> MGHHHHHHLESTSLYKKSSSTPPRGVTVVNN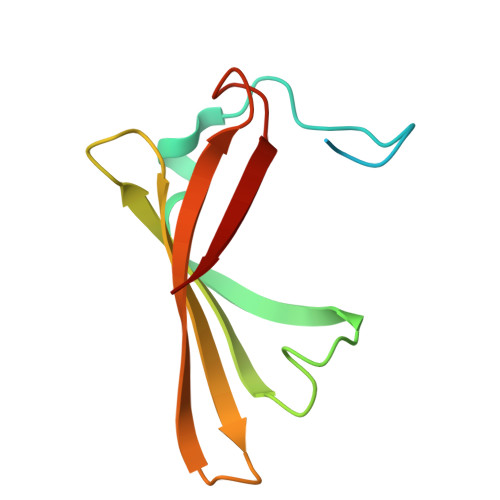FDCKRYLGTWYEIARFDHRFERGLEKVTATYSLRDDGGLNVINKGYNPDRGMWQQSEGKAYFTGAPTRAALKVSFF>MNIVAKPTSFISGAVDGVVDLKNTYTENQHLKERLEELAQLESEVADLKKENKDLKESLDITDSIRDYDPLNASVISRNPTNWNDQVEIDKGSSDGVKPDMAVTTPSGLIGKVTTTGAKSATVELLTSSDVKNRVSAKVQGKENAFGIINGYDSDTKLLELKQLPYDMKFKKGQKVVTSGLGGKFPAGIFIGTIEKVETDKMGLSQTAFIKPGADMYDLNHVTVLKRSAEAGTTDDD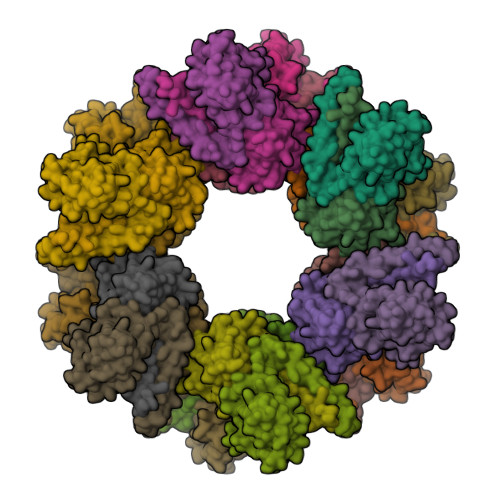TTSSDTTGGQGSHHHHHH[2x]> GSHMKNSVSVDLPGSMKVLVSKSSNADGKYDLIATVDALELSGTSDKNNGSGVLEGVKADASKVKLTISDDLGQTTLEVFKSDGSTLVSKKVTSGGSSTEEKSSGGSSEKIITRADGTRLE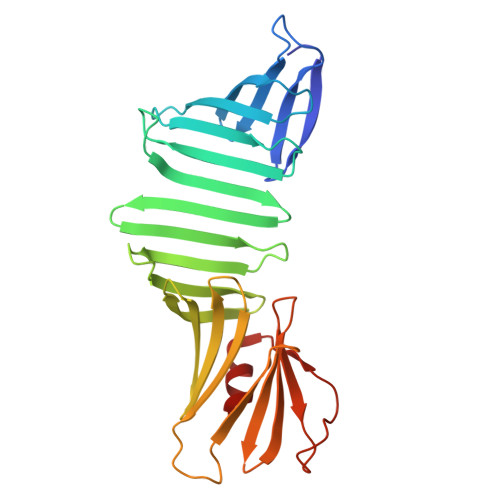YTGIKSDGSGKAKEVLKGYVLEGTLTAEKTTLVVKEGTVTLSKNISKSGEVSVELNDTDSSAATKKTAAWNSGTSTLTITVNSKKTKDLVFTSSNTITVQQYDSNGTSLEGSAVEITKLDEIKNALK> SMMIEFLNLRGKRALITAGTKGAGAATVSLFLELGAQVL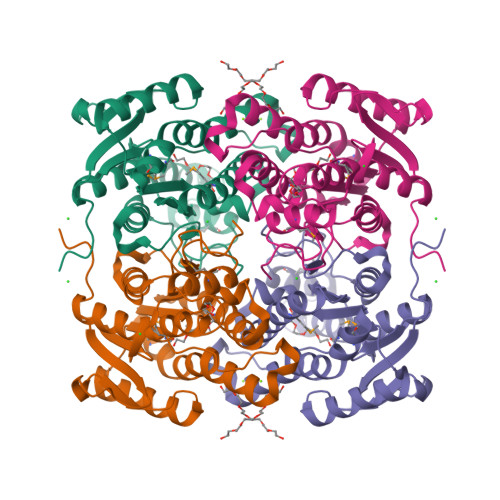TTARARPEGLPEELFVEADLTTKEGCAIVAEATRQRLGGVDVIVHMLGGSSAAGGGFSALSDDDWYNELSLNLFAAVRLDRQLVPDMVARGSGVVVHVTSIQRVLPLPESTTAYAAAKAALSTYSKAMSKEVSPKGVRVVRVSPGWIETEASVRLAERLAKQAGTDLEGGKKIIMDGLGGIPLGRPAKPEEVANLIAFLASDRAASITGAEYTIDGGTVPTA12-Amino-3-chloro-6,7,10,11-tetrahydro-5,9-dimethyl-7,11-methanocycloocta[b]quinolin-5-ium | C19 H22 Cl N2 | 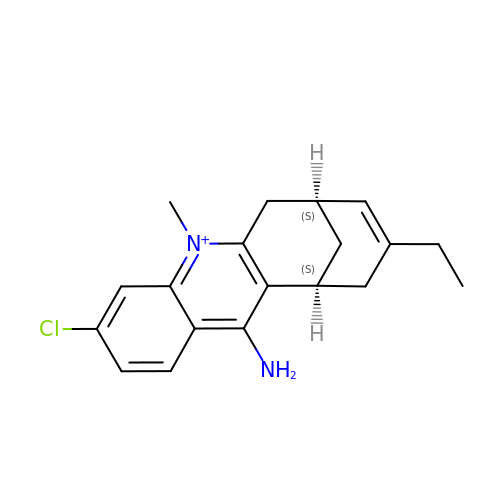UDYIKCNLONGUCX-QWHCGFSZSA-O> MSFDINWSTLESDNRLNDLIRKHLNSYLQNTQLPSYVSNLRVLDFDLGKVGPAITLKEITDPLDEFYDSIREEGGSGGSPND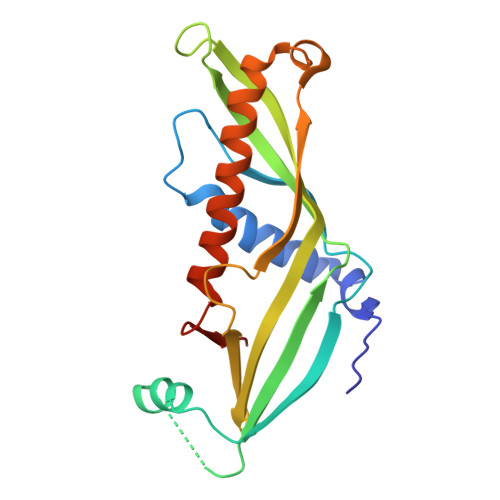IQFLLEVEYKGDLLVTIGADLVLNYPVEKFMTLPVKLSISDIGLHSLCIVACLSKQLFLSFLCDGGSIVRSMKIETEIGEQYQGQGSVLRSVGELEQFLFTIFKDFLRKELAWPSWINLDFNDGDE>[4x]AEAGITGTWYNQLGSTFIVTAGADGALTGTYESAVGNAESRYVLTGRYDSAPATDGSGTALGWTVA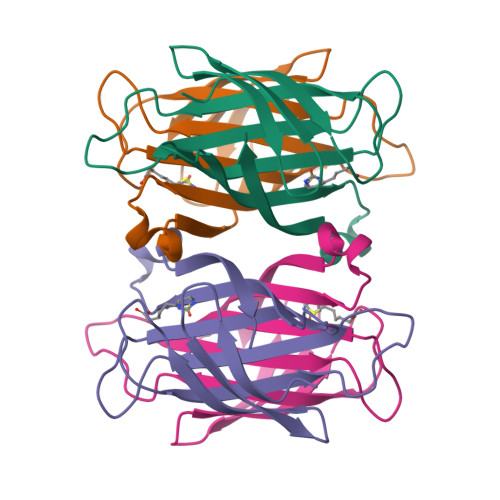WKNNYRNAHSATTWSGQYVGGAEARINTQWLLTSGTTEANAFKSTLVGHDTFTKVKPSAAS Glutamyl-tRNA synthetase (GluRS) is essential for tRNA aminoacylation and is under investigation as a bacterial drug target. GluRS catalyzes tRNA aminoacylation: the binding of glutamate to tRNA. The structures of Elizabethkingia GluRSs reported here share ∼97% sequence identity. EmGluRS and EaGluRS are monomeric enzymes that assemble with a prototypical GluRS topology with an N-terminal tRNA synthetase class I (E and Q) catalytic domain and a C-terminal anticodon-binding domain.

EmGluRS was co-crystallized with glutamate, while EaGluRS is an apo structure. E. anopheles was initially isolated from Anopheles mosquitoes and causes respiratory-tract illnesses in adults and neonatal meningitis in premature infants, with a notable outbreak in 2016 in Wisconsin. The EmGluRS and EaGluRS structures are very similar and have a root-mean-squared difference of ∼1.3 Å for the alignment of all main-chain Cα atoms. Intriguingly, the glutamate-binding cavity has been probed to develop promising inhibitors for Pseudomonas aeruginosa GluRS (PaGluRS; Hu et al., 2015). PaGluRS has a similar structural topology to EaGluRS and EmGluRS.

> MAHHHHHHMEKVRVRFAPSPTGPLHLGGVRTALYDYLFAKHNGGDFILRIEDTDTQRYVPGSEEYIMEALEWIGMVPDESPKHGGPYAPYRQSERRDIYDRYTEQILKTDYAYLAFDTPEELDQIRAEFEARGDVFAYNYETRNRLRNSISLPEEEVKKLLEEKTPYVIRFKMPLDRIINLNDIIRGKFSVNTNTLDDKVLVKNDGMPTYHFANIIDDHEMKITHVIRGEEWLPSMALHVLLYEAMGWDAPEFAHLSLILKPEGKGKLSKRDGDKFGFPVFPLNFTDPATGNTSAGYREEGYLPEAFINMVAMLGWSPADNKEIVSMDEMIKEFDLNKVHKAGARFSAEKAKWFNQQYLQLMSNEAILPEFKKVLAENNVEVSDEKALKIIGLMKERATFVKDIYNDGKFFFHAPESFDEKASKKAWSPETAVLMQELTEAISSLDFKAEIIKESIHHLAEAKGLGMGKVMMPLRLSLVGELKGPDVPDLMEMIGKEETISRINKAIETLK Very recently, an orphan RNA motif called NMT1 present in proteobacteria was identified to bind xanthine which is an oxidization product generated during purine degradation in purine metabolism. Bacterial RNAs containing the NMT1 motif turn off gene expression upon ligand sensing, likely by regulating translation initiation. Members of this riboswitch class respond to high concentrations of oxidized purines and they regulate genes predominantly associated to purine transport and oxidation, thus avoiding the deleterious effects of accumulation of purine degradation products in the cell. Overall, the riboswitch exhibits a rod-like, continuously stacked fold composed of three stems and two internal junctions.

Here, we describe the 2.7 Å resolution structure of NMT1 RNA in complex with xanthine. The RNA folds in a rod-like compact helical scaffold (‘I-shape’), in which the three stems exhibit co-axial stacking mediated by the junctional segments. Xanthine is bound at the intersection of J1, J2 and stem P1, where it is bracketed by the two strands of J1 and sandwiched by the terminal base pair A6-U41 of stem P1 and the base tiers formed with the nucleotides from J1 and J2. The bound xanthine is stacked between two base triples, namely A39–G35–C11 and A6–U41–A9. Xanthine itself is also engaged in a triple furnished together with G10 and U40. Further, both U40 and G10 use their Watson-Crick faces to form two hydrogen bonds with the minor groove edge of xanthine and two hydrogen bonds with the Watson-Crick edge of xanthine respectively. M2 is located in the corner between the Hoogsteen edge and the Watson-Crick edge of xanthine, and importantly, coordinates directly to the O6 atom of xanthine. M3 is located along the minor groove edge of xanthine and forms inner-sphere coordination with the phosphate of A38 (the terminal residue of stem P2a). M4 is facing the Hoogsteen edges of G35 and xanthine but is not engaged in direct interactions with xanthine. The three metal ion-relying interactions are key for shaping the binding pocket to guarantee high ligand specificity.

>GAGUAGAAGCGUUCAGCGGCCGAAAGGCCGCCCGGAAAUUGCUCC[2x]>[4x]GHMGKPDISAKDLRNIMYDHLPGFGTAFHQLVQVICKLGKDSNSLDIIHAEFQASLAEGDSPQCALIQITKRVPIFQDAAPPVIHIRSRGDIPRACQKSLRPVPPSPKIDRGWVCVFQLQDG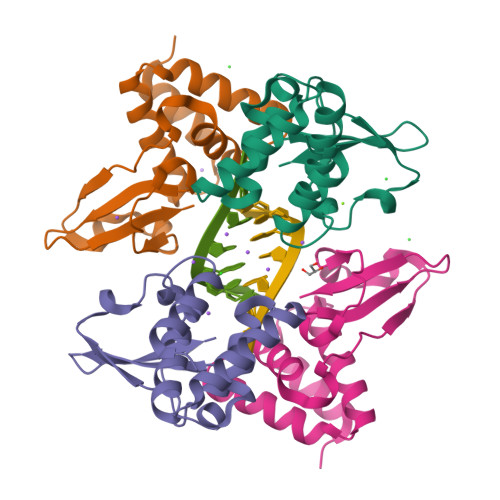KTLGLKI Anchoring of these surface proteins to the cell wall peptidoglycan requires transpeptidase enzymes called sortases, a product of an srt (surface protein sorting) gene. The membrane-associated sortase recognizes the LPXTG motif of the substrate protein, cleaves between the Thr and Gly, and forms an acyl-enzyme intermediate. According to the current model of sortase-mediated pilus assembly, the pilus polymerization catalyzed by a pilus-specific sortase is followed by cell wall anchoring of pilus polymers by the housekeeping sortase. To understand the molecular basis of pilin sorting and pilus anchoring within a bacterial strain, we investigated the housekeeping sortase, GBSSrtA, and a pilus-specific sortase, GBSSrtC1, from the PI-1 pathogenicity island of S. agalactiae SAG 2603 V/R. Either GBSSrtC1 or GBSSrtC2 of this GBS strain is capable of polymerizing GBS80, the pilus shaft of the GBS PI-1 pili.

The two molecules of the dimer, related by a non-crystallographic 2-fold axis, in the asymmetric unit of both the type II and III crystals of the GBSSrtC1 display the typical sortase fold made of an eight-stranded beta-barrel. The barrel core is flanked by two long N-terminal helices (H1 and H2), positioned approximately at 75° to each other and away from the dimer interface, which is formed by β6 strands and β4/β5 loops. Subtle differences, such as one single-turn α-helix in the β1/β2 loop present only in chain B of both dimers, and a four-turn and two-turn H1 helix in the type III and II structures, respectively, may explain the plasticity in the sortase structural features, the presence of multimers in the asymmetric unit and the observed multiple crystal-packing arrangements. Residues 44–55 and 44–54 in type II (A and B chains, respectively) and 44–51 and 46–53 in type III (chain A and B, respectively), which cover the putative active site from one-end to the other, form the lid region in GBSSrtC1. Despite the high flexibility and temperature factors (80–100 Å2), residues 46–51 were consistently positioned in all four of the active sites. Analogous to the Asp58, Pro59 and Trp60 residues of the conserved DP(W/F/Y) motif in SPNSrtC1, Asp49, Pro50 and Tyr51 of GBSSrtC1 anchored the lid in its active site. In addition, the preceding leucine residue (Leu47) was observed inserted into a highly hydrophobic pocket in the active site present below the lid. The residues in the hydrophobic pocket included Val118 (on the β4 strand), Ile162 (at the edge of the β6 strand) and Tyr171 (on the β6/β7 loop). The three catalytic residues Cys184, His122 and Arg193 of GBSSrtC1 and the corresponding residues of SPNSrtC1 (chain A) displayed similar spatial arrangements; Cys184 and Arg193 were present on the β7 and β8 strands, respectively, whereas His122 was on a loop extending from the β4 strand.

>[2x]MRGSHHHHHHGSSHANINAFKEAVTKIDRVEINRRLELAYAYNASIAGAKTNGEYPALKDPYSAEQKQAGVVEYARMLEVKEQIGHVIIPRINQDIPIYAGSAEENLQRGVGHLEGTSLPVGGESTHAVLTAHRGLPTAKLFTNLDKVTVGDRFYIEHIGGKIAYQVDQIKVIAPDQLEDLYVIQGEDHVTLLTCTPYMINSHRLLVRGKRIPYVEKTVQKDSKTFRQQQ> SLGIFPTV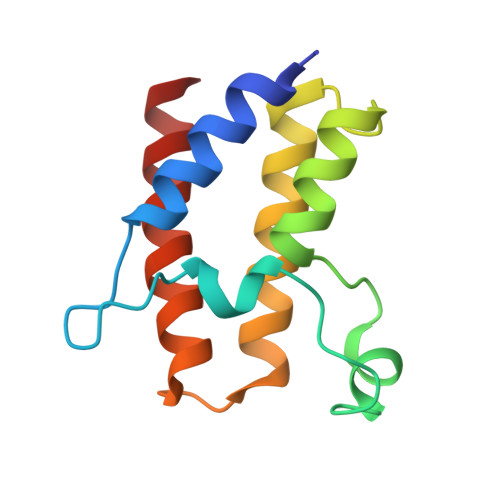EKLVEEMREQLDEVDSHPRTSIFEKLPSKRDYPDYFKVIEKPMAIDIILKNCKNGTYKTLEEVRQALQTMFENARFYNEEGSWVYVDADKLNEFTDEWFKEHSS> 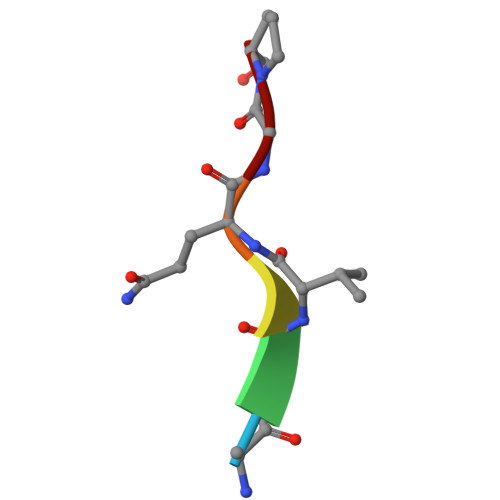AKVQGP> MG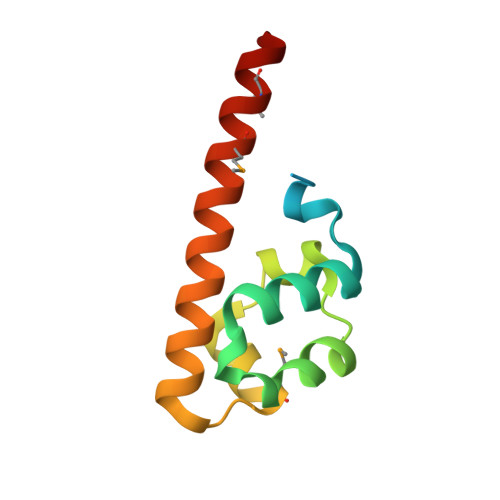EETINSTQNKTRTKTTRPKAVYLWTVSDVLKWYRRHCGEYTQYEQLFAQHDITGRALLRITDSSLQRMGVTDNRDREAIWREIVKQRLKTDIMEIRDMERLNIY> MKPEIEQELSHTLLTELLAYQFASPVRWIETQDVFLKQHNTERIIEIGPSPTLAGMANRTIKAKYESYDAALSLQRQVLCYSKDAKEIYYKPDPADLAPKETPKQEESTPSAPAAATPTPAAAAAPTPAPAPASAGPVESSSGAGSGAGAANSGGAVVDSAALDALTAENKKLAKQQLEVLARYLQVDLNKGSAKSFIKEKEASAVLQKELDLWEAEHGEFYAKGIQPTFSALKSRTYDSYWNWARQDVLSMYFDIIFGKLTSVDRETINQCIQIMNRANPTLIKFMQYHIDHCPEYKGETYKLAKRLGQQLIDNCKQVLTEDPVYKDVSRITGPKTKVSAKGNIEYEETQKDSVRKFEQYVYEMAQGGAMTKVSQPTIQEDLARVYKAISKQASKDSKLELQRVYEDLLKVVESSKEIETEQLTKDILQAATVPTTPTEEVDDPCTPSSDDEIASLPDKTSIIQPVSSTIPSQTIPFLHIQKKTKDGWEYNKKLSSLYLDGLESAAINGLTFKDKYVLVTGAGAGSIGAEILQGLISGGAKVIVTTSRFSKKVTEYYQNMYARYGAAGSTLIVVPFNQGSKQDVDALVQYIYDEPKKGGLGWDLDAIIPFAAIPENGNGLDNIDSKSEFAHRIMLTNLLRLLGAVKSKKTTDTRPAQCILPLSPNHGTFGFDGLYSESKISLETLFNRWYSEDWGSKLTVCGAVIGWTRGTGLMSANNIIAEGIEKLGVRTFSQKEMAFNILGLLTPEIVQLCQEEPVMADLNGGLQFIDNLKDFTSKLRTDLLETADIRRAVSIESAIEQKVVNGDNVDANYSKVMVEPRANMKFDFPTLKSYDEIKQIAPELEGMLDLENVVVVTGFAEVGPWGNSRTRWEMEAYGEFSLEGAIEMAWIMGFIKYHNGNLKGKPYSGWVDAKTQTPIDEKDIKSKYEEEILEHSGIRLIEPELFNGYDPKKKQMIQEVVVQHDLEPFECSKETAEQYKHEHGEKCEIFEIEESGEYTVRILKGATLYVPKALRFDRLVAGQIPTGWDARTYGIPEDTISQVDPITLYVLVATVEALLSAGITDPYEFYKYVHVSEVGNCSG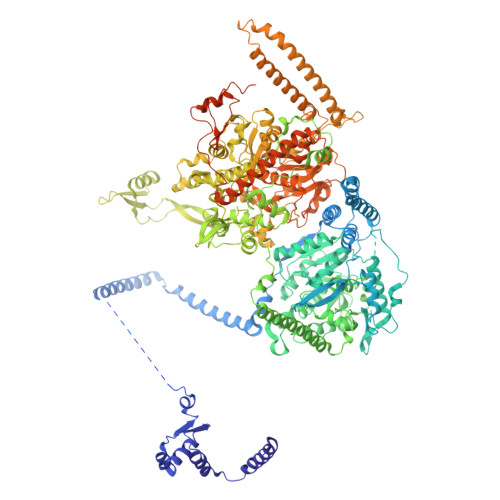SGMGGVSALRGMFKDRYADKPVQNDILQESFINTMSAWVNMLLLSSSGPIKTPVGACATAVESVDIGIETILSGKAKVVLVGGYDDFQEEGSYEFANMNATSNSIEEFKHGRTPKEMSRPTTTTRNGFMEAQGSGIQVIMTADLALKMGVPIHAVLAMTATATDKIGRSVPAPGKGILTTAREHHGNLKYPSPLLNIEYRKRQLNKRLEQIKSWEETELSYLQEEAELAKEEFGDEFSMHEFLKERTEEVYRESKRQVSDAKKQWGNSFYKSDPRIAPLRGALAAFNLTIDDIGVASFHGTSTVANDKNESATINNMMKHLGRSEGNPVFGVFQKYLTGHPKGAAGAWMLNGAIQILESGLVPGNRNADNVDKLLEQYEYVLYPSRSIQTDGIKAVSVTSFGFGQKGAQAVVVHPDYLFAVLDRSTYEEYATKVSARNKKTYRYMHNAITRNTMFVAKDKAPYSDELEQPVYLDPLARVEENKKKLVFSDKTIQSSQSYVGEVAQKTAKALSTLNKSSKGVGVDVELLSAINIDNETFIERNFTGNEVEYCLNTAHPQASFTGTWSAKEAVFKALGVESKGAGASLIDIEITRDVNGAPKVILHGEAKKAAAKAGVKNVNISISHDDFQATAVALSEF> GPKLSLIKVVNGCRLGKIQNLGKAGDCTVDIPGCLLYTRTGSAPHLTHQTLRNIHGVPGIAQLTLSSLAEHHEVLAEYKKGVGSFIGMPESLFYCSLHDPVTPGPAGYVTSKSVSVWGFGGRVEMTVSKFMAIQEA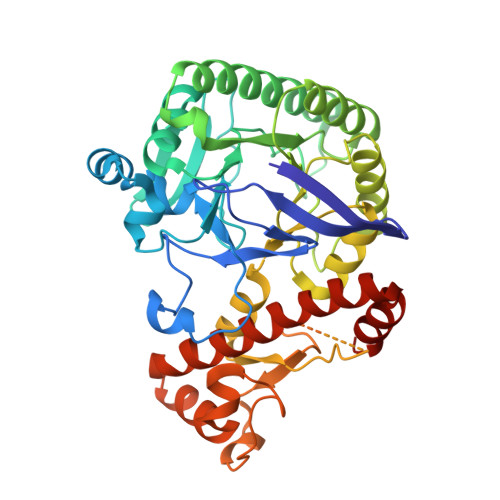LQPDWFQCLSDGEASCAETTSIKRARKSVDRSLLFLDSCLRLQEESEVLQKSVIIGVIEGGDVMEERLRSARETAKRPVGGFLLDGFQGDPAVTETRLHLLSSVTAELPEDKPRLICGVSRPDEVLECIERGVDLFESFFPYQVTERGCALTFTFDCQLNPEETLLQQNGIQEKIKGLDQAKKIEATGCNQEMTSFEINLKEKKYQEDFDPLVRGCSCYCCKNHTRAYIHHLLMTNELLAGVLLMMHNFEHYFGFFCSIREALKNDTLAQLKELICRQMFDNN>[3x]GPAMLPISMSDEGDSFLVK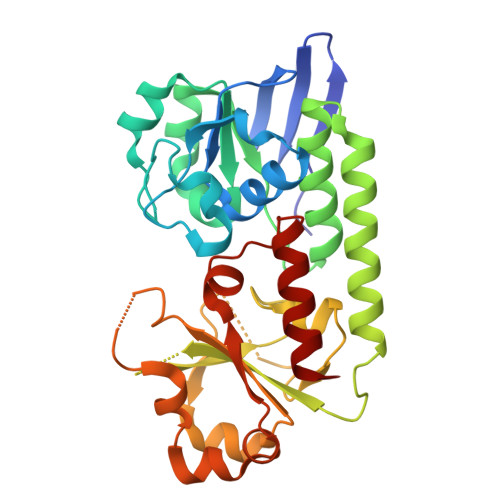DSLGENKIPKNPSKVVILDLGILDTFDALKLNDKVVGVPAKNLPKYLQQFKNKPSVGGVQQVDFEAINALKPDLIIISGRQSKFYDKLKEIAPTLFVGLDNANFLSSFENNVLSVAKLYGLEKEALEKISDIKNEIEKAKSIVDEDKKALIILTNSNKISAFGPQSRFGIIHDVLGINAVDENIKVGTLGKSINSEFILEKNPDYIFVVDRNVILGNKERAQGILDNALVAKTKAAQNKKIIYLDPEYWFLASGNGLESLKTMILEIKNAVK>[2x]GHMRGCTVWLTGLSGAGKTTVSMALEEYLVCHGIPCYTLDGDNIRQGLNKNLGFSPEDREENVRR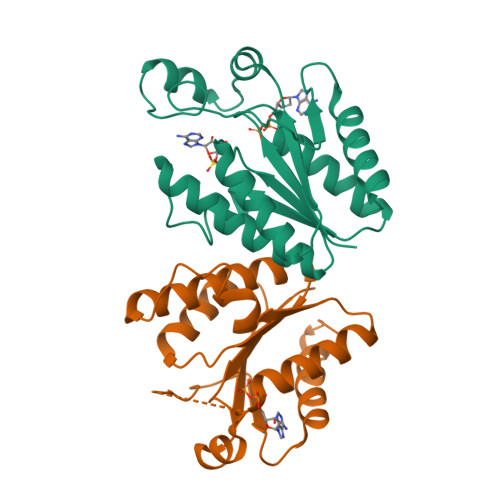IAEVAKLFADAGLVCITSFISPYTQDRNNARQIHEGASLPFFEVFVDAPLHVCEQRDVKGLYKKARAGEIKGFTGIDSEYEKPEAPELVLKTDSCDVNDCVQQVVELLQERDIV> GSHMGFRWKLAHFRYLCQSNALPSHVKINVSRQTLFEDSFQQIMALKPYDLRRRLYVIFRGEEGLDYGGLAREWFFLLSHEVLNPMYCLFEYAGKNNYCLQINPASTINPDHLSYFCFIGRFIAMALFHGKFIDTGFSLPFYKRMLSKKLTIKDLESIDTEFYNSLIWIRDNNIEECGLEMYFSVDMEILGKVTSHDLKLGGSNILVTEENKDEYIGLMTEWRFSRGVQEQTKAFLDGFNEVVPLQWLQYFDEKELEVMLCGMQEVDLADWQRNTVYRHYTRNSKQIIWFWQFVKETDNEVRMRLLQFV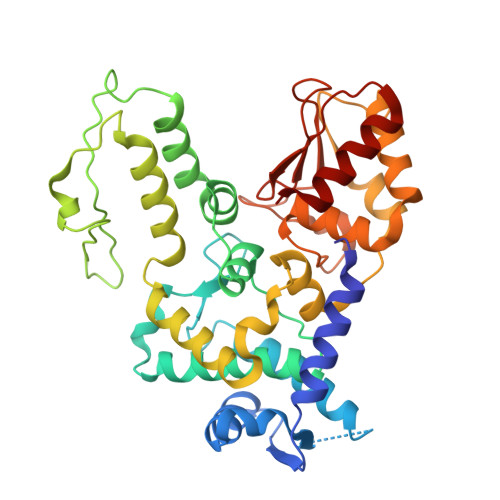TGTCRLPLGGFAELMGSNGPQKFCIEKVGKDTWLPRSHTCFNRLDLPPYKSYEQLKEKLLFAIEETE N-(2,4-dichlorobenzyl)-4-(pyrimidin-2-yloxy)piperidine-1-carboxamide 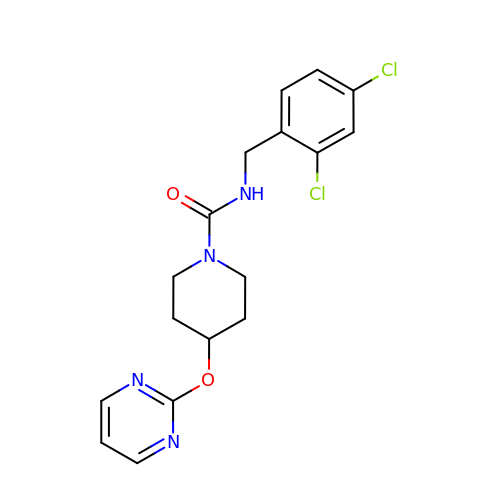| C17 H18 Cl2 N4 O2 | UZEPPAOAIDTLTK-UHFFFAOYSA-N>FASLSRFVETLVVADDKMAAFHGAGLKRYLLTVMAAAAKAFKHPSIRNPVSLVVTRLVILGSGEEGPQV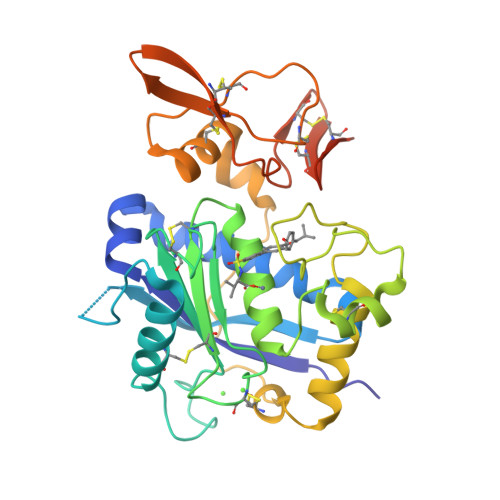GPSAAQTLRSFCAWQRGLNTPEDSDPDHFDTAILFTRQDLCGVSTCDTLGMADVGTVCDPARSCAIVEDDGLQSAFTAAHQLGHVFNMLHDNSKPCISLNGPLSTSRHVMAPVMAHVDPEEPWSPCSARFITDFLDNGYGHCLLDKPEAPLHLPVTFPGKDYDADRQCQLTFGPDSRHCPQLPPPCAALWCSGHLNGHAMCQTKHSPWADGTPCGPAQACMGGRCLHMDQLQDFNIPQADYKDDDDK[4x]>[4x]WVQPITAQKPSLTLWLDDKMFTGLINTGADVTIIK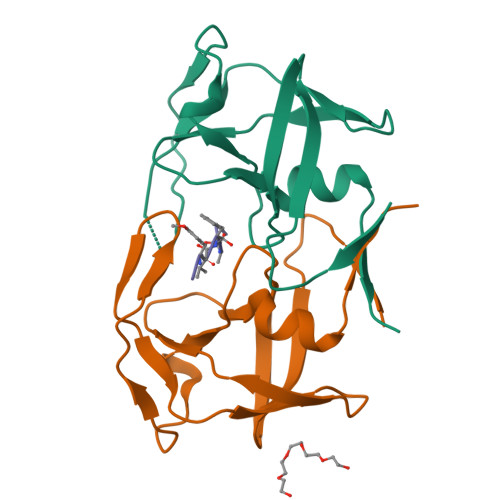LEDWPPNWPITDTLTNLRGIGQSNNPKQSSKYLTWRDKENNSGLIKPFVIPNLPVNLWGRDLLSQMKIMMASPNDIVTA;>[2x]PYVFAMT>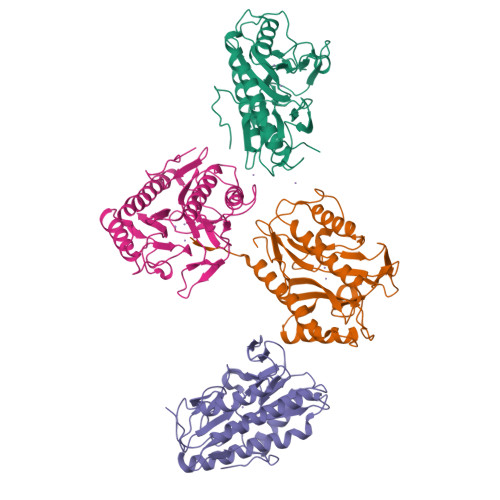[4x]MTVTIKTPDDIEKMRIAGRLAAEVLEMIGEHIKPGVTTEELDRICHDYIVNEQKAIPAPLNYKGFPKSICTSINHVVCHGIPNEKPLKEGDILNVDITVIKDGYHGDTSKMFLVGKTPEWADRLCQITQECMYKGISVVRPGAHLGDIGEIIQKHAEKNGFSVVREYCGHGIGKVFHEEPQVLHYGRAGTGIELKEGMIFTIEPMINQGRPETRLLGDGWTAITKDRKLSAQWEHTVLVTADGYEILTLRNDETFPRTSAAEFELVDKLAAALEHHHHHH>SNAGNNDLENVKAIAIVYRELSDGSQTVLLAKMKGLADEKGWMFVRGHVRKDEEADPGVAAIRETQ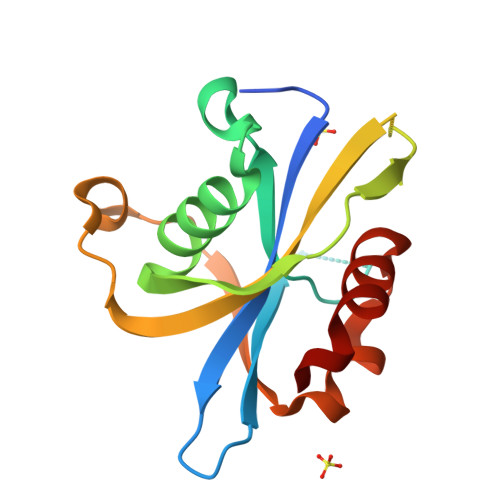EETGFTGMVKQSGAPFTQPGSKDPQRVITIHPHIVQVQEASKSKDTEDTVKREFLWVRPSEVRSKLQRAEMIQAWDQLHSFF[2x]4-(dimethylamino)-N-{4-[(3S)-3-({4-[(8R)-2-phenylpyrazolo[1,5-a]pyridin-3-yl]pyrimidin-2-yl}amino)pyrrolidine-1-carbonyl]phenyl}butanamide | C34 H36 N8 O2 | 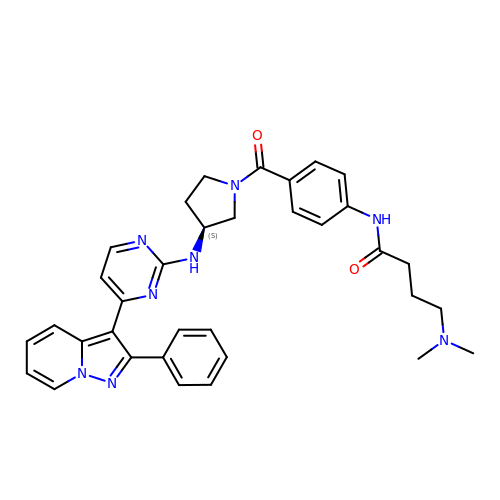HDSKLOGUAXMLMX-MHZLTWQESA-N>[4x]SNAQPEFDRGFLRPFGAKMKFLKPDQVQKLSTDDLITYMAEKDKNVRDLAIKLRDAKQDSTKNGTPEIKQKYDKAYEKTKAAAEKLVSEESLTRDALLELTEEQYVEKAALFDKDVYRNN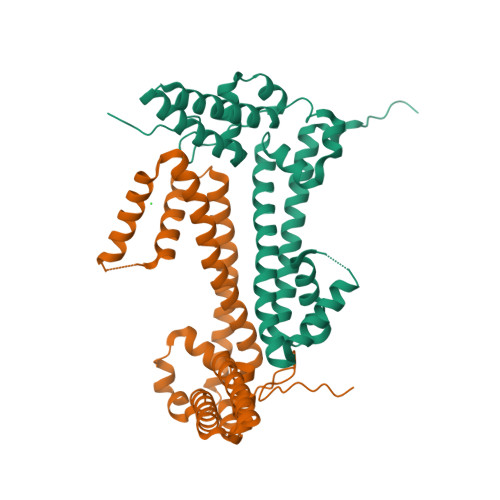LQRQTYERLLRSETDVSYREVARTFIAREGEPALNAKIERLALTLENNADTRSKLDYLAIAADFLKNQANLHADDPELNLYKAETKAREIKANRAMKEALEGADKLFERNKILKSPDM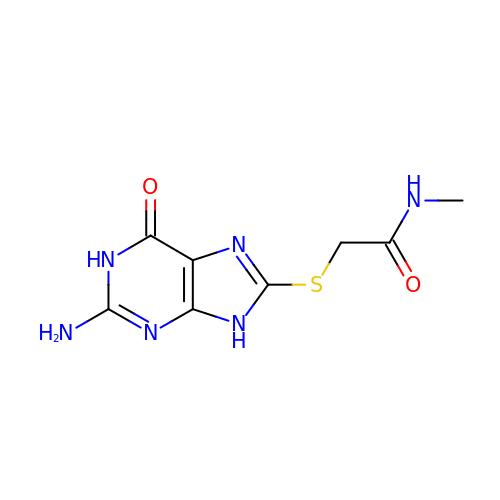2-[(2-amino-6-oxo-6,9-dihydro-1H-purin-8-yl)sulfanyl]-N-methylacetamide | C8 H10 N6 O2 S | MKEVUZQIEYSSFO-UHFFFAOYSA-N> DLPDVQELITQVRSEKCSLQAAAILDANDAHQTETSSSQVKDNKPLVERFETFCLDPSLVTKQANLVHFPPGFQPIPCKPLFFDLALNHVAFPPLEDKLAAATKSG;> MASGGSGGVSVPALWSEVNRYGQNGDFTRALKTVNKILQINKDDVTALHCKVVCLIQNGSFKEALNVINTHTKVLANNSLSFEKAYCEYRLNRIENALKTIESANQQTDKLKELYGQVLYRLERYDECLAV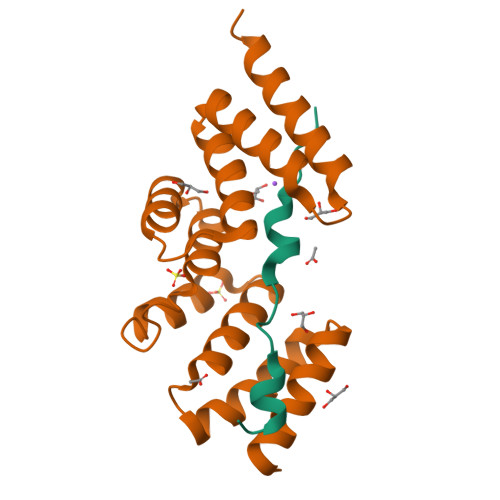YRDLVRNSQDDYDEERKTNLSAVVAAQSNWEK> MRETDEEPEEPGRRGSFVEMVDNLRGKSGQGYYVEMTVGSPPQTLNILVDTGSSNFAVGAAPHPFLHRYYQRQLSSTYRDLRKGVYVPYTQGKWEGELGTDLVSIPHGPNVTVRANIAAITESDKFFINGSNWEGILGLAYAEIARPDDSLEPFFDSLVKQTHVPNLFSLQLCGAGFPLNQSEVLASVGGSMIIGGIDHSLYTGSLWYTPIRREWYYEVIIVRVEINGQDLKMDCKEYNYDKSIVDSGTTNLRLPKKVFEAAVKSIKAASSTEKFPDGFWLGEQLVCWQAGTTPWNIFPVISLYLMGEVTNQSFRITILPQQYLRPVEDVATSQDDCYKFAISQSSTGTVMGAVIMEGFYVVFDRARKRIGFAVSACHVHDEFRTAAVEGPFVTLDMEDC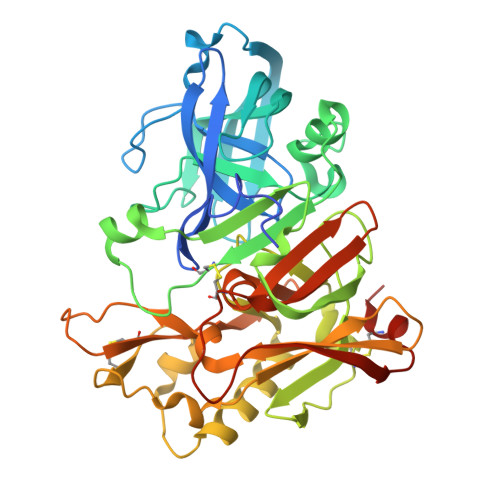GYNIPQTDEST> EQQRFPQRYIELAIVVDHGMYTKYSSNFKKIRKRVHQMVSNINEMCRPLNIAITLALLDVWSEKDFITVQADAPTTAGLFGDWRERVLLKKKNHDHAQLLTDTNFARNTIGWAYVGRMCDEKYSVAVVKDHSSKVFM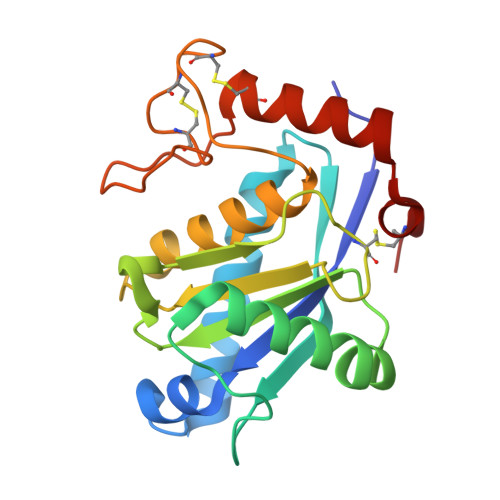VAVTMTHELGHNLGMEHDDKDKCKCTTCIMSAVISDKQSKLFSDCSKDYYQTFLTNDNPQCILNAP>[5x]GHFSVLLDVKHFSPEEIAVKVVGEHVEVHARHEERPDEHGFVAREFHRR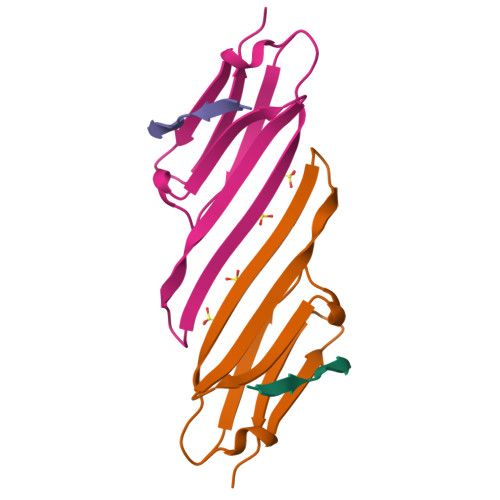YRLPPGVDPAAVTSALSPEGVLSIQAAPA;>EIPVPVQPS[5x]>[4x]GSAAAGHRTVYLFDRREKESELGDRPLQVGERSDYAGFRACVCQTLGISPEEKFVITTTSRKEITCDNFDETVKDGVTLYLLQSVNQLLLTATKERIDFLPHYDTLVKSGMYEYYASEGQNPLPFALAALIDNSLSATSRNIGVRRIQIKLLFDETQGKPAVAVIDNGRGMTSKQLNNWAVYRLSKFTRQGDFESDHSGYVRPVPVPRSLNSDISYFGVGGKQAVF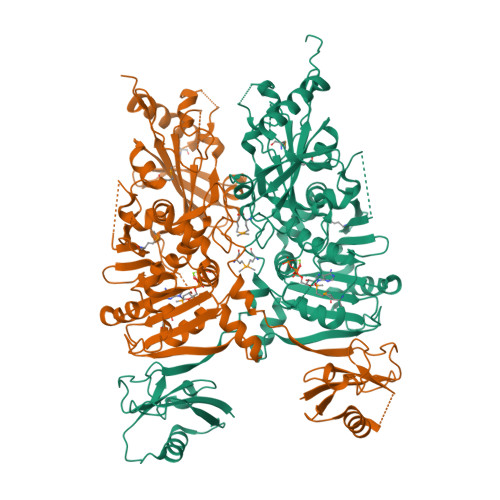FVGQSARMISKPADSQDVHELVLSKEDFEKKEKNKEAIYSGYIRNRKPSDSVHITNDDERFLHHLIIEEKEKDSFTAVVITGVQPEHIQYLKNYFHLWTRQLAHIYHYYIHGPKGNEIRTSKEVEPFNNIDIEISMFEKGKVPKIVNLREIQDDMQTLYVNTAADSFEFKAHVEGDGVVEGIIRYHPFLYDRETYPDDPCFPSKLKDEDDEDDCFILEKAARGKRPIFECFWNGRLIPYTSVEDFDWCTPPKKRGLAPIECYNRISGALFTNDKFQVSTNKLTFMDLELKLKDKNTLFTRILNGQEQRMKIDREFALWLKDCHEKYDKQIKFTLFK>[2x]MGSSHHHHHHSSGLVPRGSTDDGEKYSTVERAVKSVDPPATFKPKDEQVFYPNGKPNHQFLKQHFIHEGRLHEHQAIQILKQATHLLSKEPNLLSVPAPVTICGDVHGQYYDLMKLFEVGGDPASTKYLFLGDYVDRGSFSIECLLYLYSLKINYPDTFWMLRGNHECRHLTEYFTFKNE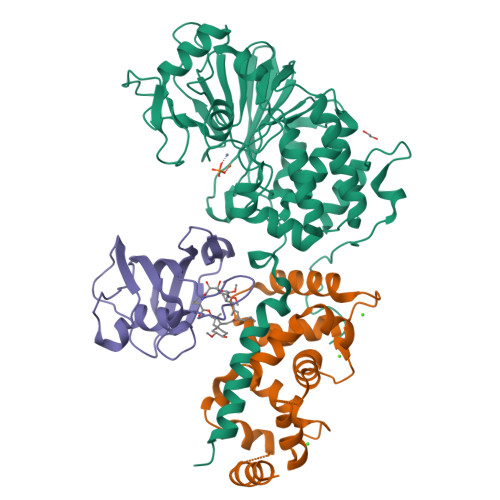CLHKYSEELYEECLVSFNALPLAAIMNEQFFCVHGGLSPQLTSLDSLRKLHRFREPPTKGLMCDLLWADPIEEYDDDNLDQEYVTNVVRGCSFAFTYKAACKFLDRTKLLSVIRAHEAQNAGYRMYKRTKTMGFPSLLTMFSAPNYLDSYNNKAAVLKYENNVMNIRQFNASPHPYWLPHFMDVFTWSLPFVGEKVTDMLVSILNVCTEEELDEDLPFSEAEIGVTPTTTT;>[2x]MGANASILDGFIEDTNFSIEEIDRLRKRFMKLDKDGSGQIDKQEFLSIPGISSNPLATRLMDVFDKDGDGSIDFEEFITGLSAFSGKSDNLNKLRFAFNIYDIDRDGYIGNGELFIVMKMMVGKNLKDEELQQIVDKTLMEADLDGDGKLNFEEFKNAVNTDTIANTLTLNMF;>[2x]GSHMSEELPQIEIVQEGDNTTFAKPGDTVTIHYDGKLTNGKEFDSSRKRGKPFTCTVGVGQVIKGWDISLTNNYGKGGANLPKISKGTKAILTIPPNLAYGPRGIPPIIGPNETLVFEVELLGVNGQ>[4x]MAAACRSVKGLVAVITGGASGLGLATAERLVGQGASAVLLDLPNSGGEAQAKKLGNNCVFAPADVTSEKDVQTALALAKGKFGRVDVAVNCAGIAVASKTYNLKKGQTHTLEDFQRVLDVNLMGTFNVIRLVAGEMGQNEPDQGGQRGVIINTASVAAFEGQVGQAAYSASKGGIVGMTLPIARDLAPIGIRVMTIAPGLFGTPLLTSLPEKVCN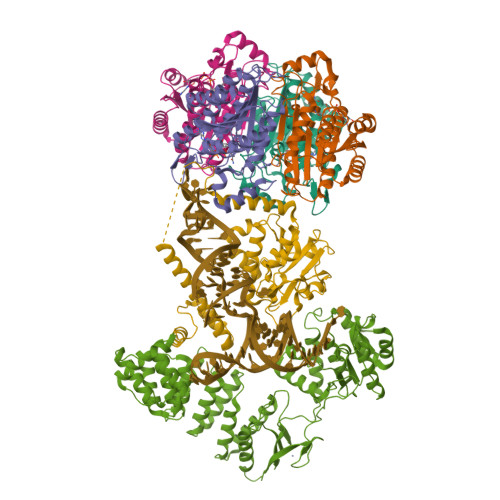FLASQVPFPSRLGDPAEYAHLVQAIIENPFLNGEVIRLDGAIRMQP;> SNAFSLKTMSPQNTKATNLIAKARYLRKDEGSNKQVYSVPHFFLAGAAKERSQMNSQTEDHALAPVRNTIQLPTQPLNSEEWDKLKEDLKENTGKTSFESWIISQMAGCHSSIDVAKSLLAWVAAKNNGIVSYDLLVKYLYLCVFHMQTSEVIDVFEIMKARYKTLEPRGYSLLIRGLIHSDRWREALLLLEDIKKVITPSKKNYNDCIQGALLHQDVNTAWNLYQELLGHDIVPMLETLKAFFDFGKDIKDDNYSNKLLDILSYLRNNQLYPGESFAHSIKTWFESVPGKQWKGQFTTVRKSGQCSGCGKTIESIQLSPEEYECLKGKIMRDVIDGGDQYRKTTPQELKRFENFIKSRPPFDVVIDGLNVAKMFPKVRESQLLLNVVSQLAKRNLRLLVLGRKHMLRRSSQWSRDEMEEVQKQASCFFADDISEDDPFLLYATLHSGNHCRFITRDLMRDHKACLPDAKTQRLFFKWQQGHQLAIVNRFPGSKLTFQRILSYDTVVQTTGDSWHIPYDEDLVERCSCEVPTKWLCLHQKT;> SNAMSSKIPAVTYPKNESTPPSEELELDKWKTTMKSSVQEECVSTISSSKDEDPLAATREFIEMWRLLGREVPEHITEEELKTLMECVSNTAKKKYLKYLYTKEKVKKARQIKKEMKAAAREEAKNIKLLETTEEDKQKNFLFLRLWDRNMDIAMGWKGAQAMQFGQPLVFDMAYENYMKRKELQNTVSQLLESEGWNRRNVDPFHIYFCNLKIDGALHRELVKRYQEKWDKLLLTSTEKSHVDLFPKDSIIYLTADSPNVMTTFRHDKVYVIGSFVDKSMQPGTSLAKAKRLNLATECLPLDKYLQWEIGNKNLTLDQMIRILLCLKNNGNWQEALQFVPKRKHTGFLEISQHSQEFINRLKKAKT> SNAMTLTALNAISPIDGRYVNKTRALSPYFSEFALTYYRLMVEIKWFESLAANDTIPEVPALDNKARKFLSD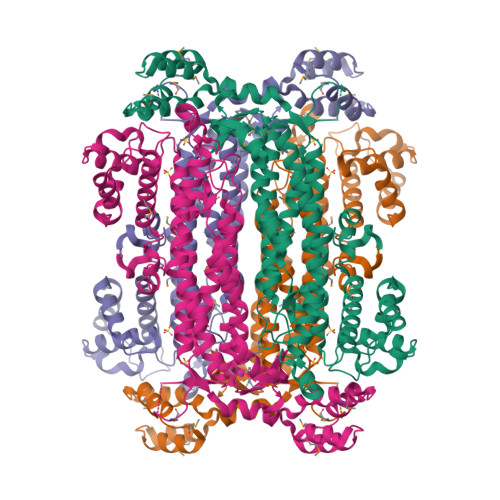LISNFNESEAEKIKEFEKQTNHDVKAVEYYLQDKFQENEQLKSCVAFIHFACTSEDINNLAYALMIKQAIAQVIQPTIAEIMGSITLLGKQHADVAMLSRTHGQPATPTTMGKELVNFVARLKRPQQQLAEVLIPAKFNGAVGNYNAHVAAYPEVDWRKHCANFVTSLGLSFNAYTTQIEPHDGIAEVSQIMVRINNILLDYTQDIWSYISLGYFKQKTIAEEVGSSTMPHKVNPIDFENAEGNLGLSNALFIHFANKLTQSRMQRDLSDSTVLRNLGVAFSYSLIAYHSVAKGNDKLQINKSALQKDLSENWEVLAEAIQTVMRRYNEPNAYEQLKELTRGQMIDAENLKKFIKTLSIPEEAKAELMKLTPETYTGLATQLVKAFS>[2x]MGSSHHHHHHSSGLVPRGHMSLFHLIAPSGYCIKQHAALRGIQRLTDAGHQVNNVEVIARRCERFAGTETERLEDLNSLARLTTPNTIVLAVRGGYGASRLLADIDWQALVARQQHDPLLICGHADFTAIQCGLLAHGNVITFSGPMLVANFGADELNAFTEHHFWLALRNETFTIEWQGEGPTCRAEGTLWGGNLAMLISLIGTPWMPKIENG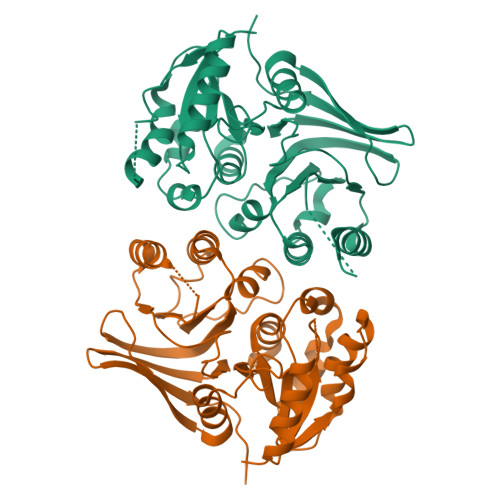ILVLEDINEHPFRVERMLLQLYHAGILPRQKAIILGSFSGSTPNDYDAGYNLESVYAFLRSRLSIPLITGLDFGHEQRTVTLPLGAHAILNNTREGTQLTISGHPVLKM>MENFPTEYFLNTTVRLLEYIRYRDSNYTREERIENLHYAYNKAAHHFAQPRQQQLLKVDPKRLQASLQTIVGMVVYSWAKVSKECMADLSIHYTYTLVLDDSKDDPYPTMVNYFDDLQAGREQAHPWWALVNEHFPNVLRHFGPFCSLNLIRSTLDFFEGCWIEQYNFGGFPGSHDYPQFLRRMNGLGHCVGASLWPKEQFNERSLFLEITSAIAQMENWMVWVNDLMSFYKEFDDERDQISLVKNYVVSDEISLHEALEKLTQDTLHSSKQMVAVFSDKDPQVMDTIECFMHGYVTWHLCDRRYRLSEIYEKVKEEKTEDAQ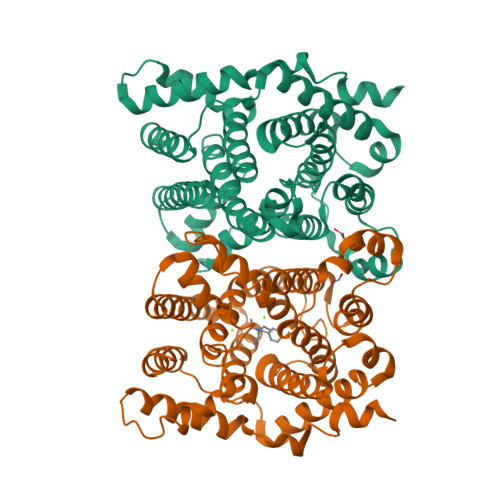KFCKFYEQAANVGAVSPSEWAYPPVAQLANVRSKDVKEVQKPFLSSIELVE[2x]>[8x]GSVDMTDNKRPQLKDKEPAAKPARTRKPKNETVALVVEATTEAEAKKSLREGGLVPAAHEIMIPVGNMILAVDTQVLDKCALALAASDDPGRWFAENESLIHSTVFAPVAKGLHRVYPLLSVRPEVPAGYEASWPTQDHMPGLHLVVGGTGAGKSSYLASQDLTLVIRWGEPAERFDV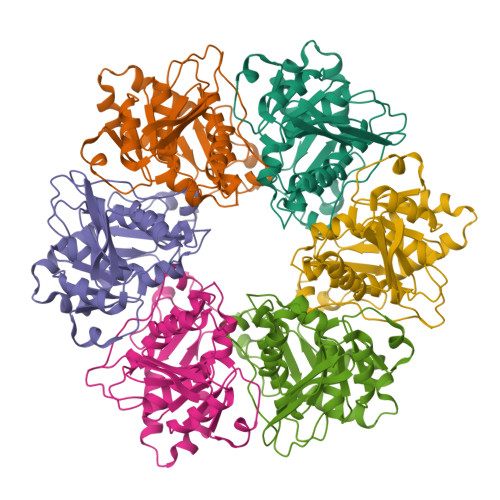EGATHAVSDLNEALAVAFVMARAGYRPAIDSFRNLVFGIESAAGEGGISTALYSAMTAINNVCSRLGIVVMVVVNPMATEAKAELVYNNMAASVAGMTVLMDGAVSKQTVRTLSGRTWGVGKQPKAAVTEEVIPRATVVPQPSAVVRNTRLESQTIDVSDDDLNNEPGRQGSRKHI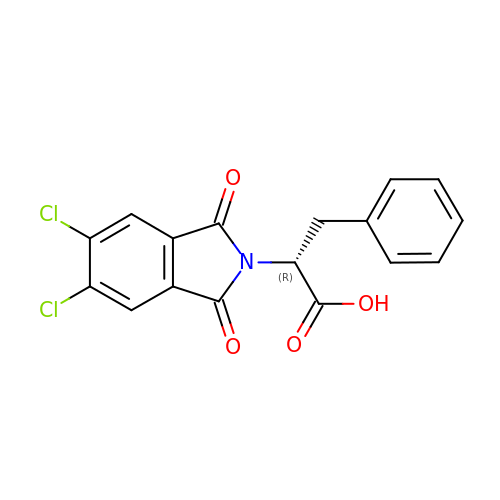(2R)-2-(5,6-dichloro-1,3-dioxo-1,3-dihydro-2H-isoindol-2-yl)-3-phenylpropanoic acid | C17 H11 Cl2 N O4 | MYKVEESSMOYIFU-CQSZACIVSA-N> SNAVDLSDADTLQRYLDQRFQQVDVSVKLELWHEAYRSIEDVFHLMKISKRAPKPSTLANYYENLVKVFFVSGDPLLHTTAWKKFYKLYSTNPRATEEEFKTYSSTIFLSAISTQLDEIPSIGYDPHLRMYRLLNLDAKPTRKEMLQSIIEDESIYGKVDEELKELYDIIEVNFDVDTVKQQLENLLVKLSSKTYFSQYIAPLRDVIMRRVFVAASQKFTTVSQSELYKLATLPAPLDLSAWDIEKSLLQAAVEDYVSITIDHESAKVTFAKDP;> MDQAVQEDFFTRLQTIIDSRGKKTVNQQSLISTLEELLTVAEKPYEFIMAYLTLIPSRFDASANLSYQPIDQWKSSFNDISKLLSILDQTIDTYQVNEFADPIDFIEDEPKEDSDGVKRILGSIFSFVERLDDEFMKSLLNIDPHSSDYLIRLRDEQSIYNLILRTQLYFEATLKDEHDLERALTRPFVKRLDHIYYKSENLIKIMETAAWNIIPAQF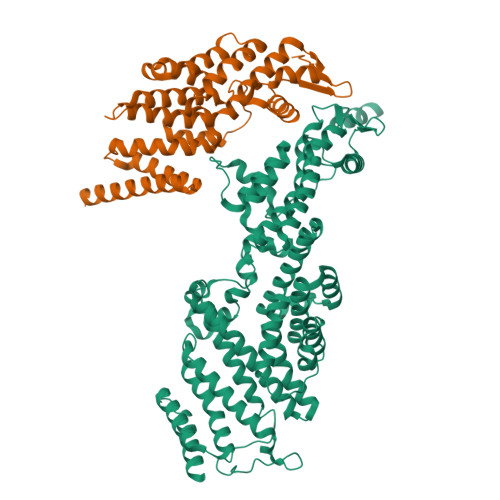KSKFTSKDQLDSADYVDNLIDGLSTILSKQNNIAVQKRAILYNIYYTALNKDFQTAKDMLLTSQVQTNINQFDSSLQILFNRVVVQLGLSAFKLCLIEECHQILNDLLSSSHLREILGQQSLHRISLNSSNNASADERARQCLPYHQHINLDLIDVVFLTCSLLIEIPRMTAFYSGIKVKRIPYSPKSIRRSLEHYDKLSFQGPPETLRDYVLFAAKSMQKGNWRDSVKYLREIKSWALLPNMETVLNSLTERVQVESLKTYFFSFKRFYSSFSVAKLAELFDLPENKVVEVLQSVIAELEIPAKLNDEKTIFVVEKGDEITKLEEAMVKLNKEYKIAKERLNPPSNRR> GLPVMNTPGSNQFLTSDDYQSPTAMPQFDVTPEMNIPGEVKNLMEIAEVDSVVPVNNVNENVNSLEAYRIPVHSVTETGAQVFGFTLQPGADTVMERTLLGEILNYYANWSGSIKLTFMYCGSAMATGKFLLAYSPPGAGVPKNRREAMLGTHIIWDIGLQSSCVLCVPWISQTHYRFVSKDIYTDAGFITC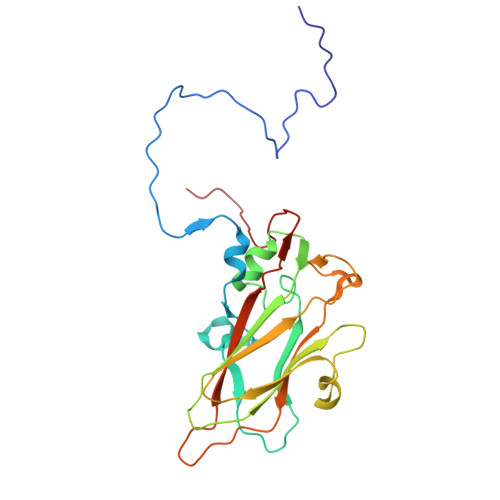WYQTSIVVPAEVQNQSVILCFVSACNDFSVRLLRDSPFVRQTAFYQ> ASADIVLFSGSKHVEFTDWGGTDWPSAYELQPPYQTMPFDLNKNFEIKVDYSGADIVLIFARWEHGSKPQIWAQ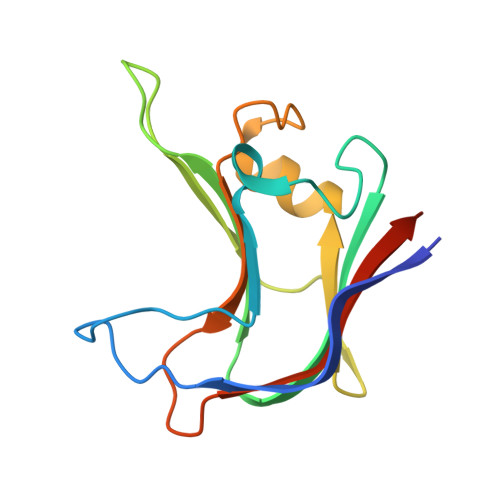ISPYYVVDGTAVFTKEQIAKAYGSDDFSDLDYIGVKPLPSADGMTVTKIVASYTSGSSDD5'-({[(2R,3S)-3-amino-4-hydroxy-2-{[2-({N-[(2R)-2-hydroxy-3,3-dimethyl-4-(phosphonooxy)butanoyl]-beta-alanyl}amino)ethyl]sulfanyl}butyl]sulfonyl}amino)-5'-deoxyadenosine 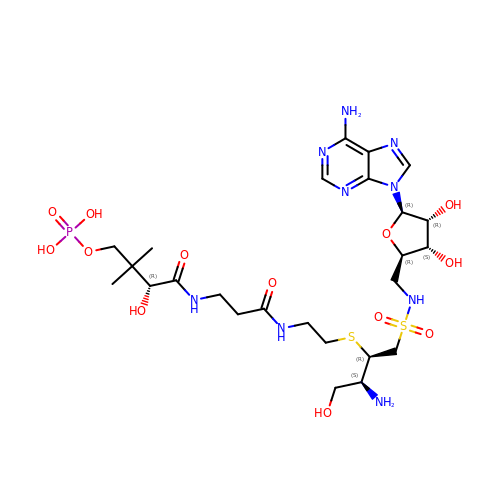| C25 H44 N9 O13 P S2 | ISNNGRBZFMWGAL-DROAMXOMSA-N> SSSHPIFHRGEFSVCDSVSVWVGDKTTATDIKGKEVMVLG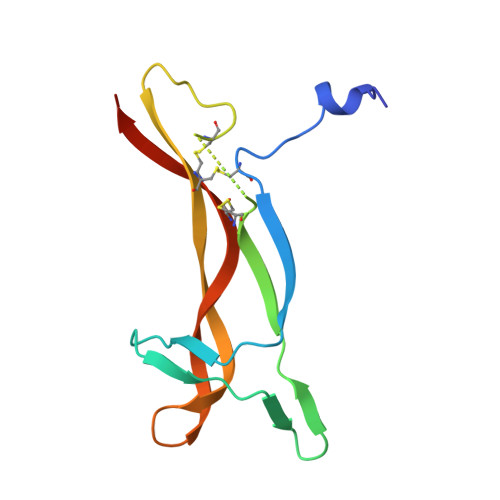EVNINNSVFKQYFFETKCRDPNPVDSGCRGIDSKHWNSYCTTTHTFVKALTMDGKQAAWRFIRIDTACVCVLSRKAVRRA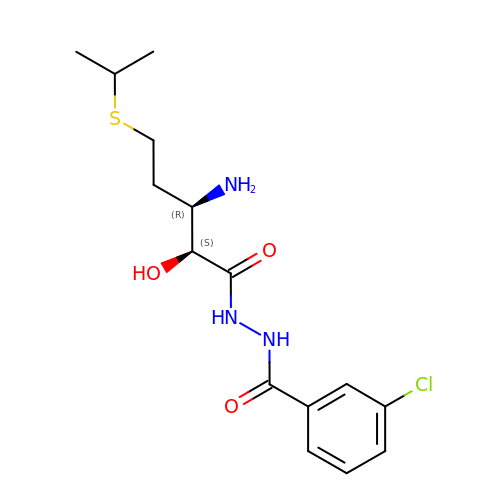N'-((2S,3R)-3-AMINO-2-HYDROXY-5-(ISOPROPYLSULFANYL)PENTANOYL)-N-3-CHLOROBENZOYL HYDRAZIDE | C15 H22 Cl N3 O3 S | BYBVYIPUGPZRSX-OLZOCXBDSA-N> PNFSGNWKIIRSENFEELLKVLGVNVMLRKIAVAAASKYAVEIKQEGDTFYIKVSTTVYTTEINFKVGEEFEEQTVDGRPCKSLVKWESENKMVCEQKLLKGEGP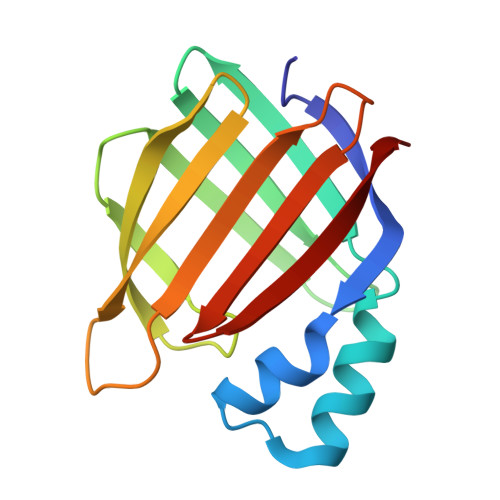KTSWTKELTNDGELIQTMTADDVVCTQVFVRE> MTHAGMKASLPNRVMLNAYPDSIDGDLAGTVRMLQRPEFTDAFGLFYVLPSIFNSDLDRGFSIIDYDLNSDLASAEDLAALDELGIMLKFDMVLNHLSVGSPQFQDLLKHGDDSAFRDFFIDWNEFWEGEGELHADGHVVPSPEHLDRLFMRKPGLPILQVRFPDGSDRFYWNTFYQRVETIDGERSYLGQMDLNAESPRVWTFYRETFEKLARYGAKIVRLDAFAYLHKAVGDTNFFNTPGTWDHLDRLRTISEENGLVLLPEIHGEYGTKIHEELSDRDYPVYDFFFPGLVIDAIDSASNTHLLRWIDEIIERDIATVNMLGCHDGIPVIDLKGGPTGQGLLPDATIEAMISRLLERGGRVKNLYGADGTKVSYYQVNATFFSALGESDARLRLARAIQLFVPGTPQVWYLDLFAGANDVEAADRAGADGHKEINRTNLSAADVEAGLARPIVLDQLEMIRLRNASPAFDGRFEVVPTDDTRLQLRWQNGSTVALLDADLATERFTITHEHDGHTEILGYDLEHHHHHH

Glycoside phosphorylases (GPs) are carbohydrate-active enzymes that catalyze the reversible cleavage of glycosidic bonds using inorganic phosphate. One of the most well-studied GPs in that regard is sucrose phosphorylase (SP; EC 2.4.1.7), which catalyzes the phosphorolysis of sucrose into α-d-glucose 1-phosphate (Glc1P) and d-fructose. Instead, a clear preference for sucrose 6F-phosphate was observed, making it the first sucrose 6F-phosphate phosphorylase (SPP; EC 2.4.1.329) ever reported. Crystal structures of the two SPPs were determined to allow for a comparison of their active site.

In this work, we report the expression and characterization of an SPP from Ilumatobacter coccineus YM16–304 (IcSPP) with active site sequence motifs that are different from the motifs found in TtSPP or in the phosphorylases with other specificities in the GH13_18 subfamily. The enzyme shows high activity on sucrose 6F-phosphate, but unlike TtSPP, it does not catalyze reactions with alternative substrates. The IcSPP crystals contained one protein molecule in the asymmetric unit, whereas the TtSPP crystals contained two. Domain A (residues 1–93, 198–328, and 389–470 in IcSPP) is the largest and forms the (β/α)8-barrel that is characteristic to the GH13 family. In IcSPP, the inner sheet immediately flanking the barrel is considerably larger and formed by three strands instead of two. IcSPP also has an additional set of two strands constituting a third, outermost β-sheet. IcSPP seems to exist as a monomer, whereas TtSPP in the crystal structure forms dimers. In IcSPP, they are found at Asp223, Glu264, and Asp327. In the structure of IcSPP, a phosphate ion is found interacting with Arg152, Glu264, Asp327, Tyr377, and Gln378 in the active site. In IcSPP, the predicted binding partners are Arg152, Glu264, Lys364, Gln378, and Lys434.>[2x]GSKAGLDQEIQEHVKKETSSEENTQKVDEHYANSLQNLAQKSLEELDKATTNEQATQVKN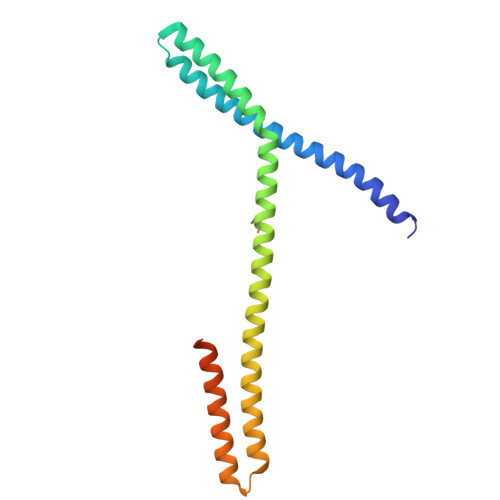QFLENAQKLKEIQPLIKETNVKLYKAMSESLEQVEKELKHNSEANLEDLVAKSKEIVREYEGKLNQSKNLPELKQLEEEAHSKLKQVVEDFRKKFKTSEQVTPKKRVKRDLA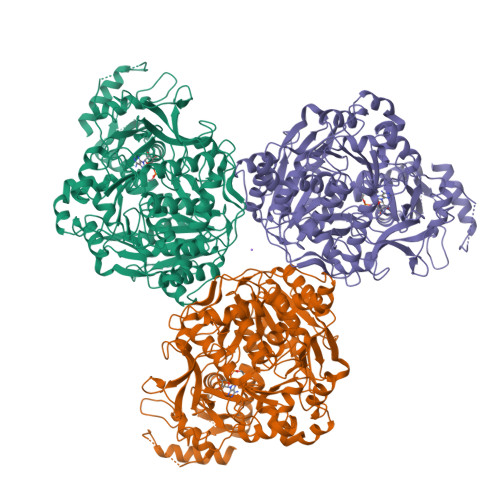> MHHHHHHHHENLYFQGPTEQTHNVVHEANGVKLRETPKEFFERQPNKGHIHDVNQYKQMYEQSIKDPQGFFGPLAKELLSWDHDFHTVKSGTLKNGDAAWFLGGELNASYNCVDRHAFANPDKPALICEADDEKDSHILTYGDLLREVSKVAGVLQSWGIKKGDTVAVYLPMNAQAIIAMLAIARLGAAHSVIFAGFSAGSIKDRVNDASCKALITCDEGKRGGRTTNIKKLCDEALVDCPTVEKVLVYKRTNNPEIHLTEGRDYYWDVETAKFPGYLPPVSVNSEDPLFLLYTSGSTGTPKGVVHSTAGYLLGAALSTKYIFDIHPEDILFTAGDVGWITGHTYALYGPLLLGVPTIIFEGTPAYPDYGRFWQIVEKHKATHFYVAPTALRLLRKAGEQEIAKYDLSSLRTLGSVGEPISPDIWEWYNEFVGKNQCHISDTYWQTESGSHLIAPLAGVVPNKPGSASYPFFGIDAALIDPVTGVEIEGNDAEGVLAIKDHWPSMARTVYKNHTKYMDTYMNPYPGYYFTGDGAARDHDGYYWIRGRVDDVVNVSGHRLSTAEIEAALIEDKKVSEAAVVGIHDDITGQAVIAYVALKEGNSDEDSEGLRKELVLQVRKTIGPFAAPKSVIIVQDLPKTRSGKIMRRILRKVSSNEADQLGDISTLSNPQSVEGIISAFGAQFGKK>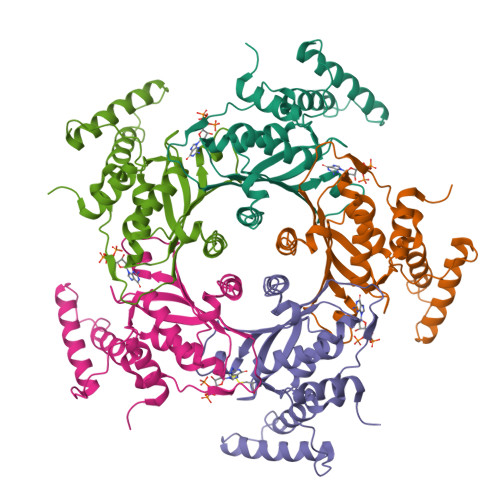[10x]PSLSKEAALVHEALVARGLETPLRPPVHEMDNETRKSLIAGHMTEIMQLLNLDLADDSLMETPHRIAKMYVDEIFSGLDYANFPKITLIENKMKVDEMVTVRDITLTSTCEHSFVTIDGKATVAYIPKDSVIGLSKINRIVQFFAQRPQVQERLTQQILIALQTLLGTNNVAVSIDAVHYCVKARGIRDATSATTTTSLGGLFKSSQNTRHEFLRAVRHHN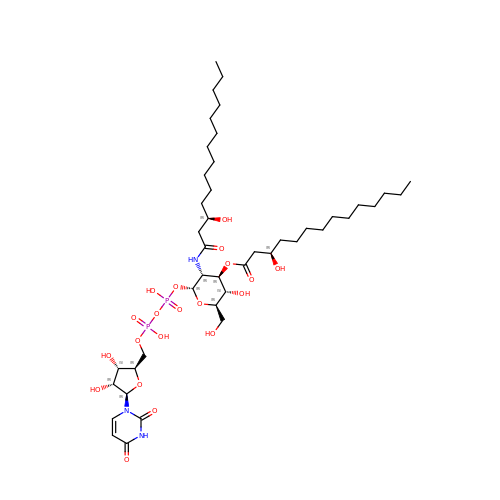(2R,3R,4R,5S,6R)-2-{[(S)-{[(S)-{[(2R,3S,4R,5R)-5-(2,4-dioxo-3,4-dihydropyrimidin-1(2H)-yl)-3,4-dihydroxytetrahydrofuran-2-yl]methoxy}(hydroxy)phosphoryl]oxy}(hydroxy)phosphoryl]oxy}-5-hydroxy-6-(hydroxymethyl)-3-{[(3R)-3-hydroxytetradecanoyl]amino}tetrahydro-2H-pyran-4-yl (3R)-3-hydroxytetradecanoate | C43 H77 N3 O20 P2 | KOJCFMYSTWNMQW-RUAJDYCTSA-N>[2x]MILDINDVLGKKIITTRLMSSITIHEENSIAALEVMSRFAADPHWLIYLPPTMSPCETSKKEGMLEHPIEAFEYFRTRGVGKVVCEQKHMGSRAVVIVCKDSQVAEKRFGVLDGTAGICYTRTGRHFFDDMQLEAELIDRVRKVLDK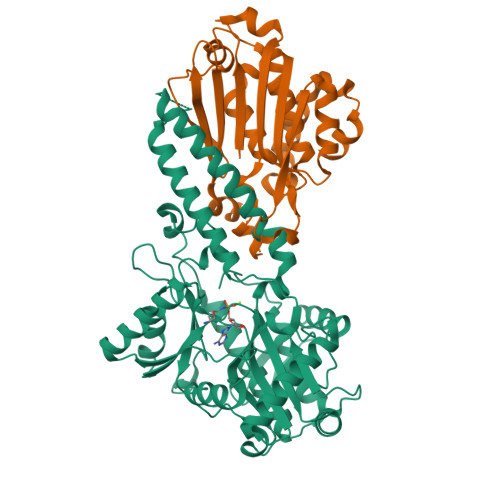SGFWGDFNTDWVCLDCELMPWSAKAQKLLEEQYSAVGISGRVVLDEAVKLLKQASLNKTVSFDVSRQTSGKNADINELLQRFTERSEMMQKYVEAYRKYCWPVNSIDDLKLAPFHILATEGKVHSDKNHIWHMDTIAKYCTQDDSLIMATNHILVDVTDAESVDKGIKWWEDLTASGGEGMVVKPYDFIVKNGRELLQPAVKCRGREYLRIIYGPEYTMDENIERLRNRAVGKKRSLALREFSLGMEALERFVRNEPLYRVHECVFGVLALESEPVDPRL;>[2x]MILTITYTQPPATDLGYLLHKNPSRPQTFELNHGKAHIFYPEATSERCTVALLLDIDPIDLARGKKGSSGEGGLFDYVNDRPYVSSSFMSVAISRVFGTAMSGKCKEKPELAAIKLPLKAKIMMLPCKGGEEIIYRLFEPLGYKVDVEGYMLDEKFPEWGKSRYYTVSLEGEVRVRDLLNHIYVLIPVLDSEKHYWVGEDEIDKLFQHGEGWLVDHPEKELITGRYLIRK>[2x]TNLRVLLDTAIPPSFCDTVSSVLLDDFNMVSLIRTSPADSLATIKQDNAEIDIAITIDEELKISRFNQCVLGYTKAFVVAHPQHPLCNASLHSIASLANYRQISLGSRSGQHSNLLRPVSDKVLFVENFDDMLRLVEAGVGWGIAPHYFVEERLRNGTLAVLSELYEPGGIDTKVYCYYNTALESERSFLRFLESARQRLREL

MvfR is a quorum sensing transcriptional regulator that regulates virulence functions critical for acute, persistent, and relapsing infections, making it a high-interest novel drug target for treatment of P. aeruginosa infections. MvfR belongs to the LysR-type transcriptional regulator (LTTR) family, which is widely conserved among prokaryotes. Two of the most abundant HAQs, namely, 4-hydroxy-2-heptylquinoline (HHQ) and 3,4-dihydroxy-2-heptylquinoline (Pseudomonas quinolone signal [PQS]), bind and activate MvfR in vivo, leading to the activation of MvfR-regulated virulence factors that promote infection. The MvfR LBD consists of two subdomains connected by an antiparallel β-sheet hinge region, with a hydrophobic ligand binding pocket between the two subdomains.

To clarify how M64 interacts with MvfR, we solved the crystal structure of the MvfR ligand binding domain (LBD) complexed with M64 (MvfRM64) using the crystal soaking methodology under the conditions reported by Ilangovan et al.. The structure of MvfRM64 was determined in the orthorhombic space group C 2 2 21 at 2.65-Å resolution, with two protein monomers in the asymmetric unit. The model comprises residues Thr93 to Leu295. M64 was found to bind to the hydrophobic pocket where 2-nonyl-4-quinolone (NHQ), a congener of the MvfR native ligands PQS and HHQ, also binds. Although M64 has a higher molecular weight than native agonists, it is able to fit into the hydrophobic pocket owing to a bend at its central sulfur atom. The overall structure of a single domain of MvfRM64 was compared and found to be similar to the crystal structures of both the MvfR LBD complexed with NHQ (MvfRNHQ) and its ligand-free form (MvfRapo) determined by Ilangovan et al., suggesting that there is no major conformational change in MvfR when it is bound by M64 relative to when it is bound by a native ligand. However, a subtle local conformational change was found in the region of helices α2 and α3 (residues 181 to 191) adjacent to the binding pocket of MvfRM64. The Leu183 residue shifts down by 3.4 Å and rotates by 180° to make direct hydrophobic contact with M64. Given a distance of less than 3.5 Å between donor and acceptor atoms, a specific hydrogen bond with a 2.99-Å distance between M64 and an oxygen atom in the side chain of Gln194 was identified with well-defined electron density. In addition, PoseView analysis revealed that the phenoxy group of M64 forms a pi interaction with the side chain of Tyr258.>[2x]GMSDPAGKPCIICVAITGSLPTKENNPAVPITLAEQVESTHEAFEAGASIAHCHVRDDEGRPTSDPDRFAALKEGLERHCPGMIVQLSTGGRSGAGQARGAMLPLCPDMASLSVGSNNFPTRVYENPPDLVDWLAAEMLKYDIKPEIEAFDLSHILQAKRMAGDGRLAGTPYVQFVMGVRNAMPADRDVF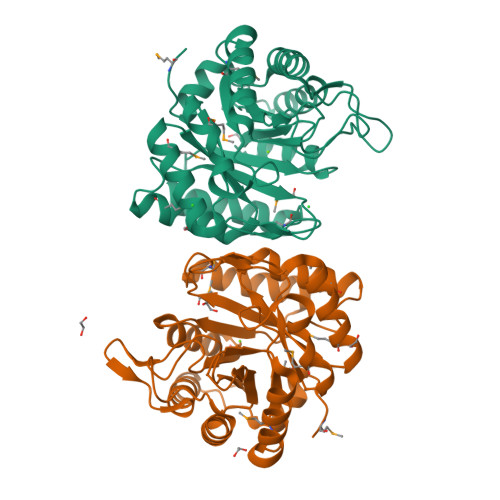DYYIHTVRRLFGEDAPWCAAGIGPSQIVLNEWAISSGGHARTGLEDNVRLDRDRLAPSNAALVGRAVELCEKYERPVATWRQARQILGLRMV4-[5-(2,6-dioxo-1,2,3,6-tetrahydropyridin-4-yl)-1H-1,2,4-triazol-3-yl]-6-oxo-1,6-dihydropyridine-2-carbonitrile | 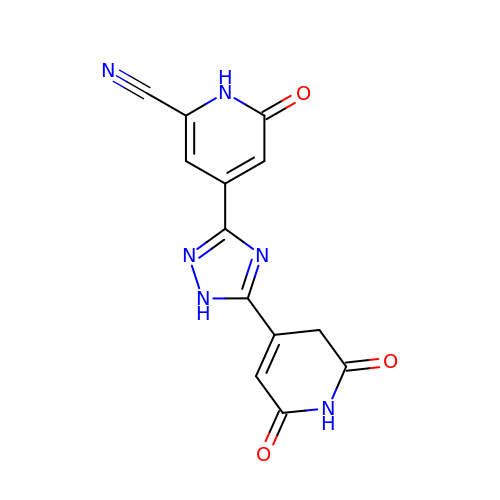C13 H8 N6 O3 | YUNURAZDMHEFGV-UHFFFAOYSA-N> GDNKINGSFDDTVKEYDFQKYTTNFETIQKGIYFNYDWGEGTTWPWQTFQNLNHDMFSGYFHDFASKFSDKNTVYALEAGWTASAWNYTYNYIFPV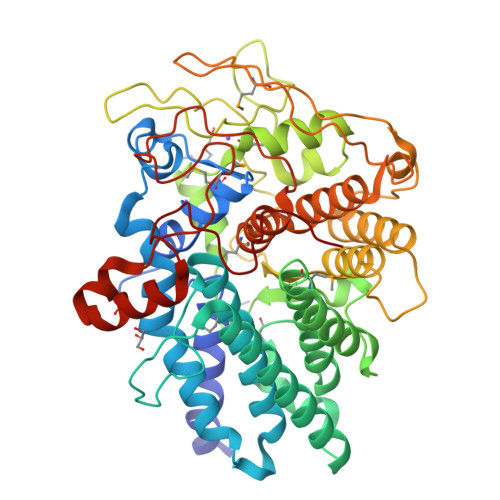AHKSTLITQDEAKYKHFYGATLILKVEAMHRITDTYGPIVYSKFGKNETNSVDTQEEAYKAFFDDLDKAVDALDTYLKEGGKEDGVKSINMCNCPTASRWIKFANSLRLRLAMRVSNVDKTLATSEAQKALENSYGVIESSDENIQISGKGYQNPLAGVAGWGETYMGATIASVLNGYEDPRISIYYNPATLAEHTEEYLGVPQGVYAKDGDPNYYQSYSFINTQTITASTPAVLLTAAETWFLRAEASLRGINPKNESAKQCYEAGVQTSFSQWGAGDASLYLTSKGKPTDYINYAAGPGKDMKALITTTPNFDDAVNQEEQLEKIITQKWIACWPEGMEAWAEQRRTGYPKLFKVQTNNSNGTIDTDIMIRRLPFSQDDAKKDPEQYKNLCTALGGADNGGTRLWWDTGKNNF> GKHTVPYTISVDGITALHRTYFVFPENKKVLYQEIDSKVKNELA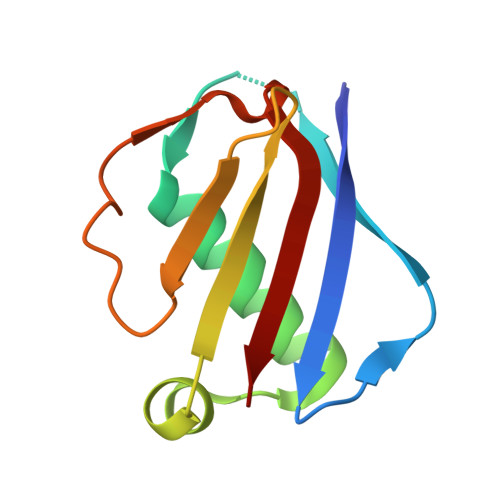SQRGVTTEKINNAQTATYTLTLNDGNKKVVNLKKNDDAKNSIDPSTIKQIQIVVK> VIGDLKCTTVSINDVDTGVPSISTDV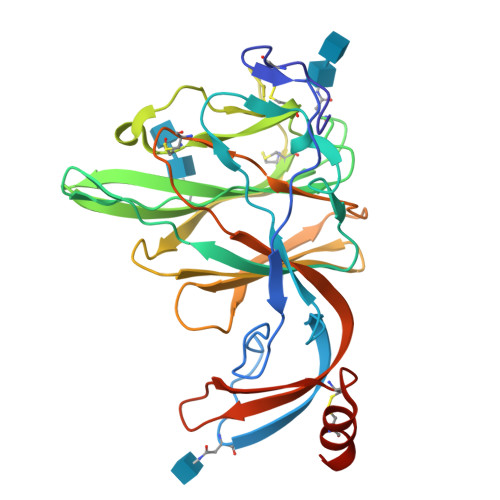VDVTNGLGTYYVLDRVYLNTTLLLNGYYPTSGSTYRNMALKGTLLLSTLWFKPPFLSDFTAGIFAKVKNTKVVKSGVTYSEFPAITIGSTFVNTSYSVVVQPHTTNLDNKLQGLLEISVCQYTMCEYPNTICHPNLGNQRVELWHWDTGVVSCLYKRNFTYDVNADYLYFHFYQEGGTFYAYFTDTGVVTKFLFNVYLGTVLSHYYVMPLTCNSAMTLEYWVTPLTSKQYLLAFNQDGVIFNAVDCKSDFMSEIKCKTHHHHHH Here, X-ray crystallography, site-directed mutagenesis and enzymatic activity data are used to define the three-dimensional structure, acceptor/donor substrate binding, membrane binding and catalytic mechanism of PatA from M. smegmatis. PatA catalyses an essential step in the biosynthesis of PIMs in M. tuberculosis. The enzyme transfers a palmitoyl moiety from palmitoyl–CoA to the 6-position of the Manp ring linked to 2-position of myo-inositol in PIM1 or PIM2. Our results reveal that the enzyme has an α/β architecture and shares with other important eukaryotic/prokaryotic acyltransferases an acid/base catalytic mechanism involving conserved histidine and aspartic/glutamic acid residues.

Two other crystal forms were obtained in P 21 (PatA–C16-2) and P 42212 (PatA–C16-3) space groups, and the corresponding crystal structures solved at 2.90 and 2.43 Å resolution, respectively, by using molecular replacement methods. The high quality of the electron density maps allowed the trace of residues 41 to 302 (PatA–C16-1), 48 to 295 (PatA–C16-2) and 48 to 303 (PatA–C16-3). We have decided to use the PatA–C16-1 crystal form for our description since it displays the highest resolution. A close inspection of the three crystal structures revealed that the protein crystallized as a monomer, displaying a high degree of structural flexibility in the N- and C-terminal regions (coloured in green in Supplementary Fig. 3; root-mean-square deviation (r.m.s.d.) value of 1.6 and 8.4 Å for Cα atoms in 41–47 and 288–302 residue ranges for the N and C terminus, respectively). Strikingly, one molecule of palmitic acid was unambiguously identified in the difference electron density maps of PatA–C16-1, PatA–C16-2 and PatA–C16-3 crystal structures. We believe that acyl molecule is associated to the enzyme due to the hydrolysis of palmitoyl–CoA during the isolation and purification of PatA from M. smegmatis mc2155. The acyl chain is deeply buried into the hydrophobic pocket, and oriented with the carboxylate group facing the groove and the acyl tail extending into the globular core of the monomer. Interestingly, the comparison of the three crystal structures revealed conformational flexibility in the carboxylate moiety of the palmitate, located in close proximity with the lateral chain of H126. In all crystal structures of palmitoyl–PatA and PatA–S-C16CoA complexes, the carboxylate OE2 oxygen atom of E200 was found at 2.8 Å of the ND1 nitrogen atom of the aromatic imidazole ring of the invariant H126. It is worth noting that when the individual palmitate molecules observed in the three crystal structures of palmitoyl–PatA were superimposed, they showed important structural flexibility at the carboxylate region, suggesting that the carboxylate group is not in a catalytically competent position in the crystal structures.

>[4x]MPEVVFGSVTDLGYAAGWRLVRAMPEAMAQGVFGAGARYAARNGGPEQLRRNLARVVGKPPADVPDDLIRASLASYARYWREAFRLPAMDHGRLGEQLDVIDIDHLWSALDAGRGAVLALPHSGNWDMAGVWLVQNYGPFTTVAERLKPESLYRRFVEYRESLGFEVLPLTGGERPPFEVLAERLTDNRPICLMAERDLTRSGVQVDFFGEATRMPAGPAKLAIETGAALFPVHCWFEGDGWGMRVYPELDTSSGDVTAITQALADRFAANIATYPADWHMLQPQWIADLSDERRARLGTSRHHHHHH> MDDFNNILDLLIN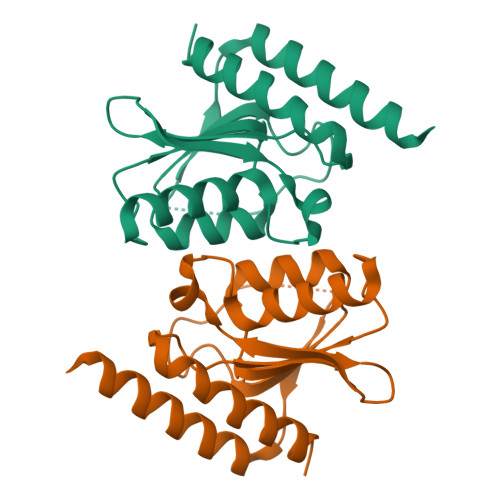ESKKAIKHNDIPVSCCIIDSNNNILSLAINSRYKNKDISQHAEINVINDLISKLNSFNLSKYKLITTLEPCMMCYSAIKQVKINTIYYLVDSYKFGIKNNYSINDQNLNLIQIKNQKKQSEYIKLLNIFFINKRLEHHHHHH>HHHHHHFNLPPGNYKKPKLLYCSNGGHFLRILPDGTVDGTRDRSDQHIQLQLSAESVGEVYIKSTETGQYLAMDTDGLLYGSQTPNEECLFLERLEENHYNTYISKKH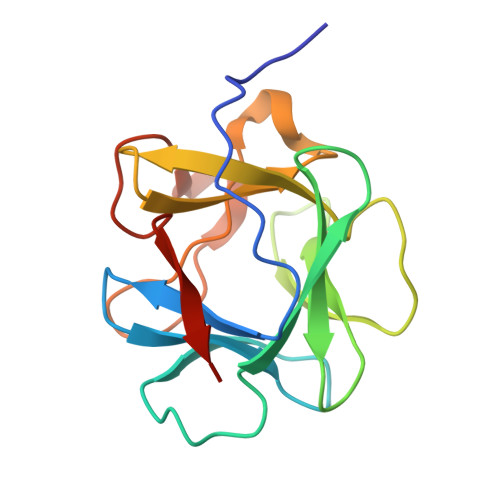AEKNWFVGLKKNGSVKRGPRTHYGQKAILFLCLPVSSD[4x]> SMVQSSGPMDVTSLTEELK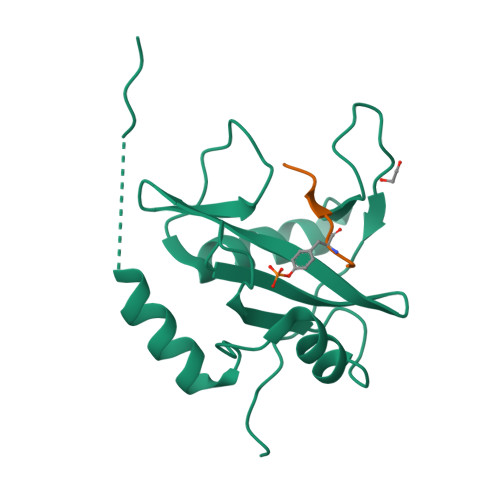KLAKQGWYWGPITRWEAEGKLANVPDGSFLVRDSSDDRYLLSLSFRSHGKTLHTRIEHSNGRFSFYEQPDVEGHTSIVDLIEHSIGDSENGAFCYSRSRLPGSATYPVRLTNPVSRFMQVRS;> NGNNYVYIDPT>MNLLRRSGKRRRSESGSDSFSGSGGDSSASPQFLSGSVLSPPPGLGRCLKAAAAGECKPTVPDYERDKLLLANWGLPKAVLEKYHSFGVKKMFEWQAECLLLGQVLEGKNLVYSAPTSAGKTLVAELLILKRVLEMRKKALFILPFVSVAKEKKYYLQSLFQEVGIKVDGYMGSTSPSRHFSSLDIAVCTIERANGLINRLIEENKMDLLGMVVVDELHMLGDSHRGYLLELLLTKICYITRKSASCQADLASSLSNAVQIVGMSATLPNLELVASWLNAELYHTDFRPVPLLESVKVGNSIYDSSMKLVREFEPMLQVKGDEDHVVSLCYETICDNHSVLLFCPSKKWCEKLADIIAREFYNLHHQAEGLVKPSECPPVILEQKELLEVMDQLRRLPSGLDSVLQKTVPWGVAFHHAGLTFEERDIIEGAFRQGLIRVLAATSTLSSGVNLPARRVIIRTPIFGGRPLDILTYKQMVGRAGRKGVDTVGESILICKNSEKSKGIALLQGSLKPVRSCLQRREGEEVTGSMIRAILEIIVGGVASTSQDMHTYAACTFLAASMKEGKQGIQRNQESVQLGAIEACVMWLLENEFIQSTEASDGTEGKVYHPTHLGSATLSSSLSPADTLDIFADL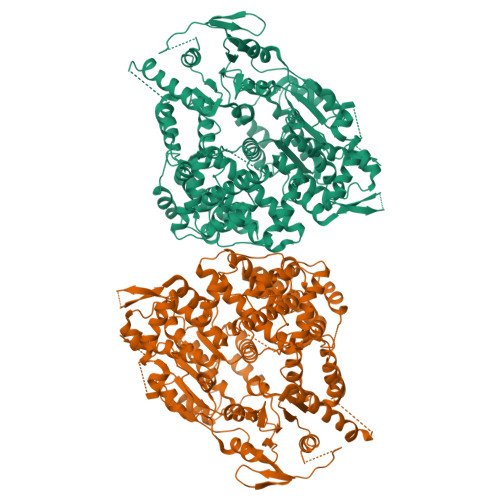QRAMKGFVLENDLHILYLVTPMFEDWTTIDWYRFFCLWEKLPTSMKRVAELVGVEEGFLARCVKGKVVARTERQHRQMAIHKRFFTSLVLLDLISEVPLREINQKYGCNRGQIQSLQQSAAVYAGMITVFSNRLGWHNMELLLSQFQKRLTFGIQRELCDLVRVSLLNAQRARVLYASGFHTVADLARANIVEVEVILKNAVPFKSARKAVDEEEEAVEERRNMRTIWVTGRKGLTEREAAALIVEEARMILQQDLVEM[2x]> AYVEIIEQPKQRGMRFRYKCEGRSAGSIPGERSTDTTKTHPTIKINGYTGPGTVRISLVTKDPPHRPHPHELVGKDCRDGYYEADLCPDRSIHSFQNLGIQCVKKRDLEQAISQRIQTNNNPFHVPIEEQRGDYDL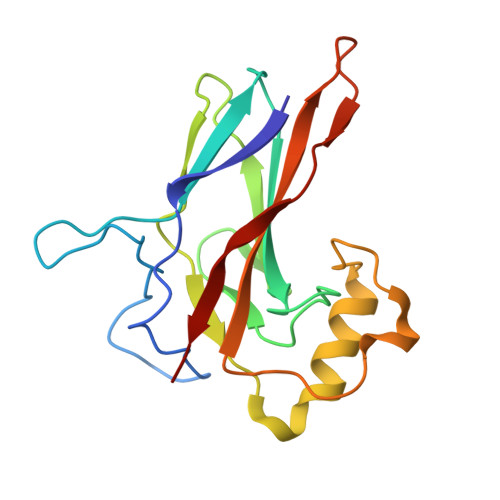NAVRLCFQVTVRDPAGRPLLLTPVLSHPIFDNRA> SLEVTEADAT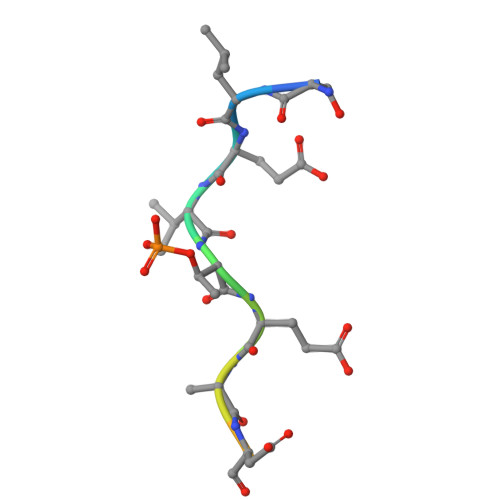FAK>MAATTENLPQLKS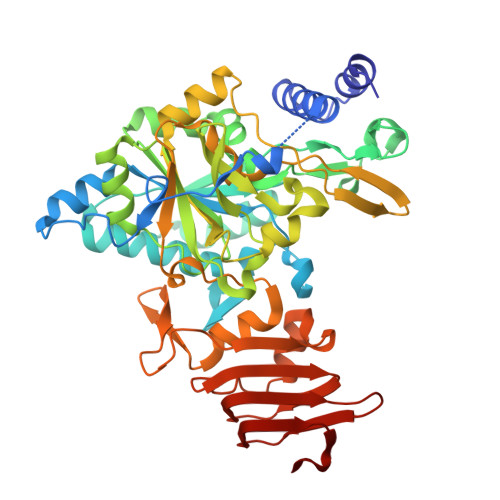AVDGLTEMSESEKSGFISLVSRYLSGEAQHIEWSKIQTPTDEIVVPYEKMTPVSQDVAETKNLLDKLVVLKLNGGLGTTMGCTGPKSVIEVRDGLTFLDLIVIQIENLNNKYGCKVPLVLMNSFNTHDDTHKIVEKYTNSNVDIHTFNQSKYPRVVADEFVPWPSKGKTDKEGWYPPGHGDVFPALMNSGKLDTFLSQGKEYVFVANSDNLGAIVDLTILKHLIQNKNEYCMEVTPKTLADVKGGTLISYEGKVQLLEIAQVPDEHVNEFKSIEKFKIFNTNNLWVNLKAIKKLVEADALKMEIIPNPKEVDGVKVLQLETAAGAAIRFFDNAIGVNVPRSRFLPVKASSDLLLVQSDLYTLVDGFVTRNKARTNPSNPSIELGPEFKKVATFLSRFKSIPSIVELDSLKVSGDVWFGSSIVLKGKVTVAAKSGVKLEIPDRAVVENKNINGPEDL[2x]>[2x]HHHHHHFNLPPGNYKKPKLLYCSNGGHFLRILPDGTVDGTRDRSDQHIQLQLSAESVGEVYIKSTETGQYLAMDTDGLLYGSQTPNSECLFLERLEEN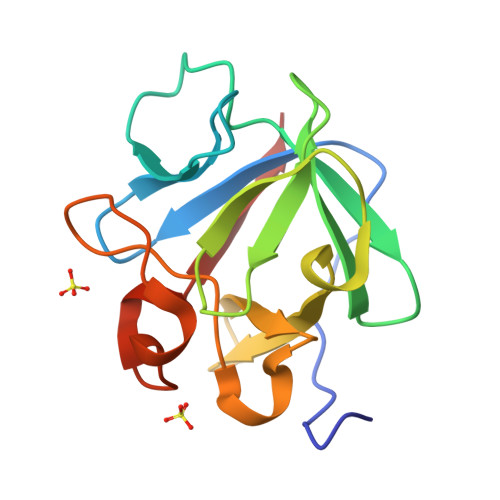HYNTYISKAHAEKNWFVGLKKNGSCKRGPRTHYGQKAILFLPLPVSSD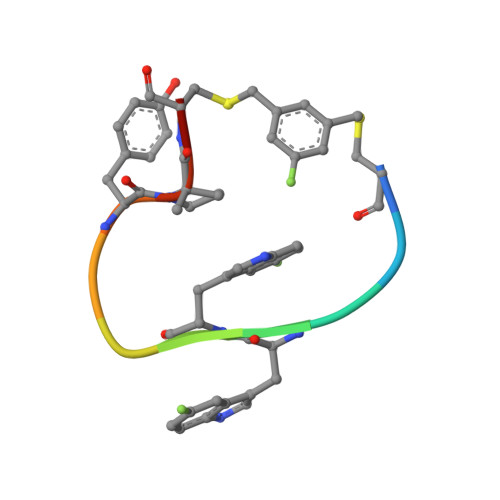> CKAWWPTYXCA>[2x]GAMGIPQHQQKHALMAIKAVKRLKDARPFLQPV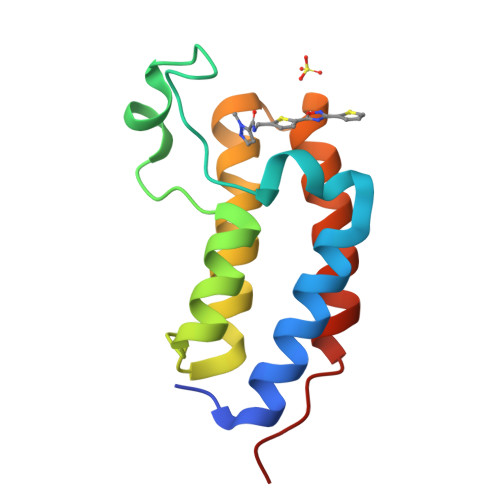DPVALNIPLYFNFIKRPMDLQTIERKLNANAYETPEQITEDFNLMVENSAKFNGPTAVITQMGRNIQAAFEKHMLNMPAKD>[2x]GAMGSFNSIDVEINMYPVNKTSCNSSIGSSSTISTSELTITLTHEDCTPVFIGDYYSVVDKLATSGFFTNDKVHQDLTTQCKINLEIKCNSGRESRQLTPTTKVYLMPHSETVTVVGDCLSNLDVYIVYANTDAIYSDMDVVAYHTSYILNVDHIPPNDCERD

In addition to the anti-TNF activity attributed to the N-terminal four cysteine-rich domains (CRDs) homologous to host TNF receptors, CrmB and CrmD have anti-chemokine activity attributed to a unique C-terminal extension (∼160 aa), named as the SECRET domain (smallpox virus-encoded chemokine receptor). Biochemical analysis revealed that the SECRET domain binds a subset of human and mouse CC, CXC and C chemokines, including CCL28, CCL25, CCL20, CXCL12, CXCL13, CXCL14, and XCL1. The identification of other poxvirus genes encoding homologues with the SECRET domain indicates that the SECRET domain represents a new family of viral CKBPs, which has specific folding to allow its binding with chemokines, either independently or fused with vTNFRs. Here we report the crystal structures of the SECRET domain of CrmD encoded by an ECTV strain and the complex of it with chemokine CX3CL1.

The crystal structure of the SECRET domain (residues S162−D320) was determined at a resolution of 1.57 Å by using single-wavelength anomalous dispersion (SAD) method with a Br-soaked derivative. There are two SECRET domains (molecules A and B) in the asymmetric unit, related by a non-symmetrical two-fold axis with an r.m.s.d. of 0.62 Å for all Cα atoms. Although these two monomers bind each other tightly with a buried surface of ∼1160 Å2, the size exclusion chromatography revealed that it is monomeric in solution. Therefore, the SECRET dimer in the asymmetric unit is caused by molecular packing and unlikely has any functional significance. The SECRET domain monomer adopts a β-sandwich fold, consisting of two parallel β-sheets and the connecting loops. The β-sheet I consists of five anti-parallel strands 1, 5, 6, 10 and 11. The β-sheet II consists of six strands, which can be further divided into two segments (antiparallel strands 2, 3, 4 and 7; antiparallel strands 8 and 9). The β-sheet II outside surface is completely exposed to solvent, whereas the solvent accessibility of β-sheet I outside surface is limited by a long C-terminal loop after strand 11 surrounding the bottom half of β-sheet I. A disulfide bond, C180−C317, further fixes the conformation of this extended loop by connecting it to the 1–2 loop. However, there are several significant differences in the arrangement of certain secondary structure elements, making the CrmD SECRET domain more compact than vCCI and A41 and also directly affecting its binding with chemokines.> GSGEGPREPGAAGGAAGGSRDALSLEEILRLYNQPIN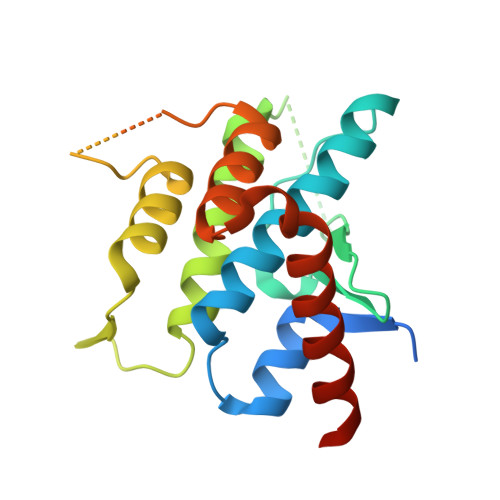EEQAWAVCYQCCGSLRAAARRRQPRHRVRSAAQIRVWRDGAVTLAPAADDAGEPPPVAGKLGYSQCMETEVIESLGIIIYKALDYGLKENEERELSPPLEQLIDHMANTVEADGSNDEGYEAAEEGLGDEDEKRKISAIRSYRDVMKLCAAHLPTESDAPNHYQAVCRALFAETMELHTFLTK> MEEPEEPADSGQSLVPVYIYSPEYVSMCDSLAKIPKRASMVHSLIEAYALHKQMRIVKPKVASMEEMATFHTDAYLQHLQKVSQEGDDDHPDSIEYGLGYDCPATEGIFDYAAAIGGATITAAQCLIDGMCKVAINWSGGWHHAKKDEASGFCYLNDAVLGILRLRRKFERILYVNLDLHHGDGVEDAFSFTSKVMTVSLHKFSPGFFPGTGDVSDVGLGKGRYYSVNVPIQDGIQDEKYYQICESVLKEVYQAFNPKAVVLQLGADTIAGDPMCSFNMTPVGIGKCLKYILQWQLATLILGGGGFNLANTARCWTYLTGVILGKTLSSEIPDHEFFTAYGPDYVLEITPSCRPDRNEPHRIQQILNYIKGNLKH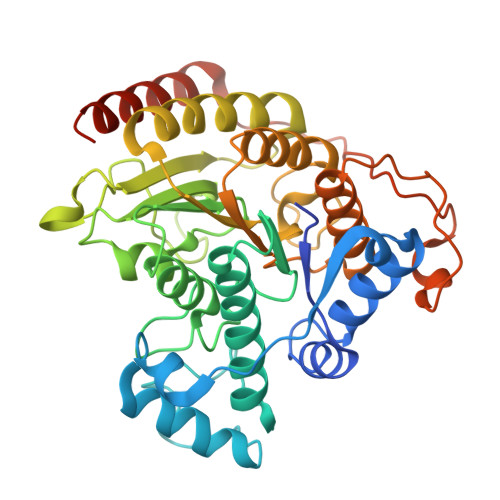VVIEGRGSHHHHHH>MASNRGQLNHELSKLFNELWDADQNRMKSGKDYRISLQGKAGYVPAGSNQARDSASFPLFQFVDEEKLKSRKTFATFISLLDNYEMDTGVAEVVTPEEIAENNNFLDAILETKVMKMAHDYLVRKNQAKPTRNDFKVQLYNIWFQLYSRAPGSRPDSCGFEHVFVGESKRGQEMMGLHNWVQFYLQEKRKNIDYKGYVARQNKSRPDEDDQVLNLQFNWKEMVKPVGSSFIGVSPEFEFALYTIVFLASQEKMSREVVRLEEYELQIV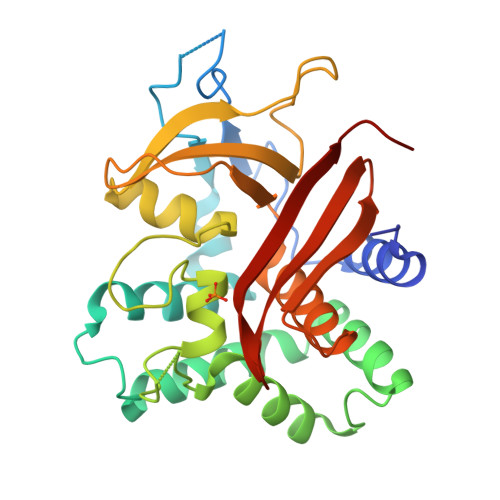VNRHGRYIGTAYPVLLSTNNPDLY[3x]>[2x]TLSILVAHDLQRVIGFENQLPWHLPNDLKHVKKLSTGHTLVMGRKTFESIGKPLPNRRNVVLTSDTSFNVEGVDVIHSIEDIYQLPGHVFIFGGQTLFEEMIDK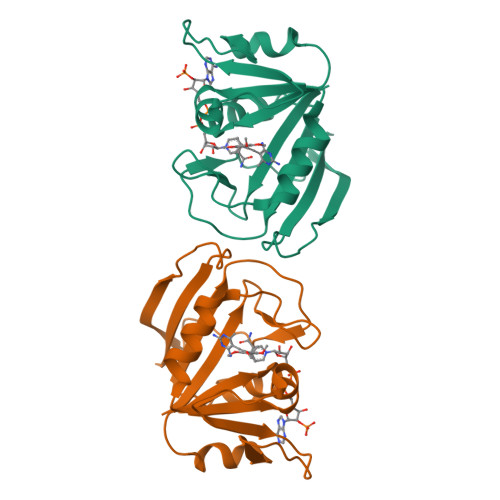VDDMYITVIEGKFRGDTFFPPYTFEDWEVASSVEGKLDEKNTIPHTFLHLIRK> EFLTAVSSIDTFLPVLNEAKLQWPTSALAASSEELLGGYVGSQFYLQDGKYMQFQIAGSSNRCELRQMIPDGGSEIGWAVDDGTTHTATSSIVVPEQVDGVEEVTIMQIHSGEAPQLRISWIRSKSL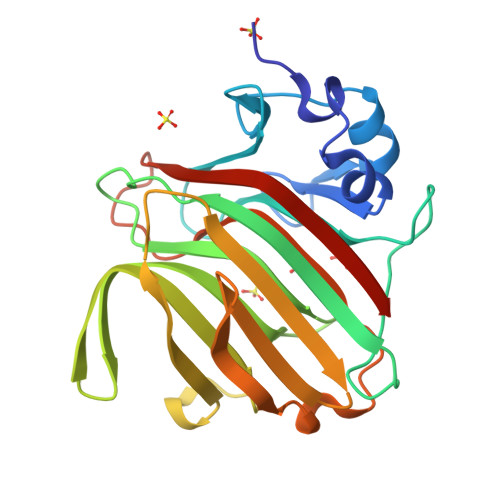DGVAYEDFIMSTVRIGTGDSSDNFVKTHLADRTAGAMSFQIDVKDSKLTITVNGNVVVNGQDLSFWDGTDSCYFKAGAYNNNPTSESATARIKFAALAWVDHHHHHH>[2x]AGLNTAAKAKGLKYFGSATDNPELTDSAYVAQLSNTDDFGQITPGNSMKWDATEPSQNSFSFANGDAVVNLANKNGQLMRCHTLVWHSQLPNWVSSGSWTNATLLAAMKNHITNVVTHYKGKCYAWDVVNEALNEDGTFRNSVFYQIIGPAYIPIAFATAAAADPDVKLYYNDYNIEYSGAKATAAQNIVKMIKAYGAKIDGVGLQAHFIVGST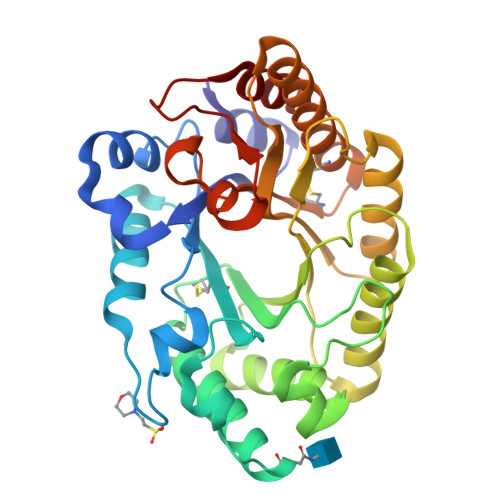PSQSDLTTVLKGYTALGVEVAYTELDIRMQLPSTAAKLAQQSTDFQGVAAACVSTTGCVGVTIWDWTDKYSWVPSVFQGYGAPLPWDENYVKKPAYDGLMAGLGA> MSQ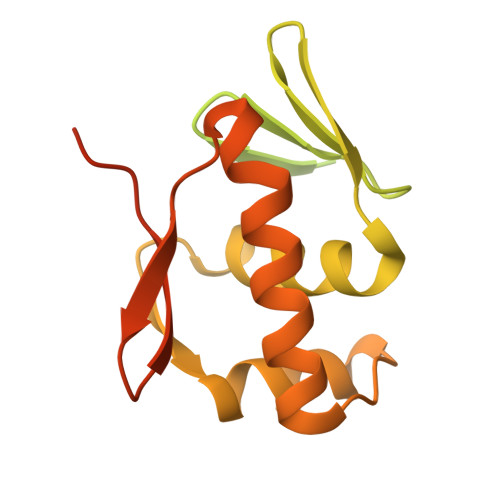EQGKIYIVEDDMTIVSLLKDHLSASYHVSSVSNFRDVKQEIIAFQPDLILMDITLPYFNGFYWTAELRKFLTIPIIFISSSNDEMDMVMALNMGGDDFISKPFSLAVLDAKLTAILRRSQQFIQQELTFGGFTLTREGLLSSQDKEVILSPTENKILSILLMHPKQVVSKESLLEKLWENDSFIDQNTLNVNMTRLRKKIVPIGFDYIHTVRGVGYLLQDPNSSSVDKLAAALEHHHHHH>SMGKLSEHLRYCDSILREMLSKKHAAYAWPFYKPVDAEALELHDYHDIIKHPMDLSTVKRKMD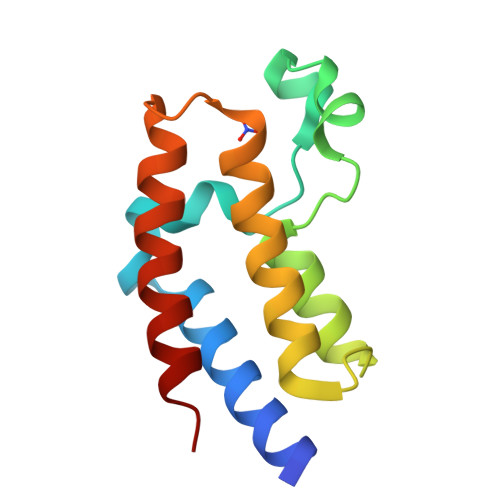GREYPDAQGFAADVRLMFSNCYKYNPPDREVVAMARKLQDVFEMRFAKMP[4x]>MSEMTPREIVSELDQHIIGQADAKRAVAIALRNRWRRMQLQEPLRHEVTPKNILMIGPTGVGKTEIARRLAKLANAPFIKVEATKFTEVGYVGKEVDSIIRDLTDSAGGAIDAVEQNGIVFIDEIDKICKKGEYSGADVSREGVQRDLLPLVEGSTVSTKHGMVKTDHILFIASGAFQVARPSDLIPELQGRLPIRVELTALSAADFERILTEPHASLTEQYKALMATEGVNIAFTTDAVKKIAEAAFRVNEKTENIGARRLHTVMERLMDKISFSASDMNGQTVNIDAAYVADALGEVVENEDLSRFIL[3x];>[6x]TTIVSVRRNGQVVVGGDGQVSLGNTVMKGNARKVRRLYNGKVLAGFAGGTADAFTLFELFERKLEMHQGHLLKSAVELAKDWRTDRALRKLEAMLIVADEKESLIITGIGDVVQPEEDQILAIGS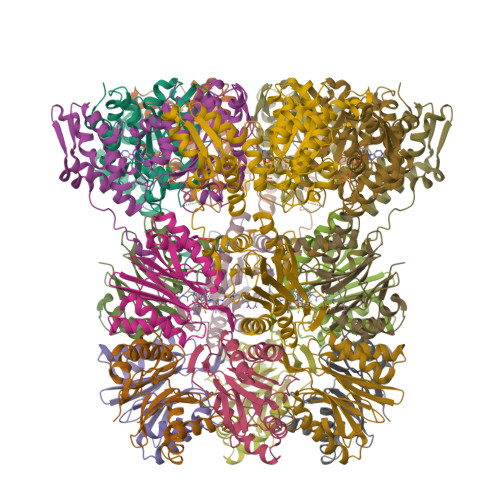GGNYALSAARALVENTELSAHEIVEKSLRIAGDICVFTNTNFTIEELPN> MSASFVPNGASLEDCHCNLFCLADLTGIKWKKYVWQGPTSAPILFPVTEEDPILSSFSRCLKADVLGVWRRDQRPGRRELWIFWWGEDPSFADLIHHDLSEEEDGVWENGLSYECRTLLFKAVHNLLERCLMNRNFVRIGKWFVKPYEKDEKPINKSEHLSCSFTFFLHGDSNVCTSVEINQHQPVYLLSEEHITLAQQSNSPFQVILCPFGLNGTLTGQAFKMSDSATKKLIGEWKQFYPISCCLKEMSEEKQEDMDWEDDSLAAVEVLVAGVRMIYPACFVLVPQSDIPTPSPVGSTHCSSSCLGVHQVPASTRDPAMSSVTLTPPTSPEEVQTVDPQSVQKWVKFSSVSDGFNSDSTSHHGGKIPRKLANHVVDRVWQECNMNRAQNKRKYSASSGGLCEEATAAKVASWDFVEATQRTNCSCLRHKNLKSRNAGQQGQAPSLGQQQQILPKHKTNEKQEKSEKPQKRPLTPFHHRVSVSDDVGMDADSASQRLVISAPDSQVRFSNIRTNDVAKTPQMHGTEMANSPQPPPLSPHPCDVVDEGVTKTPSTPQSQHFYQMPTPDPLVPSKPMEDRIDSLSQSFPPQYQEAVEPTVYVGTAVNLEEDEANIAWKYYKFPKKKDVEFLPPQLPSDKFKDDPVGPFGQESVTSVTELMVQCKKPLKVSDELVQQYQIKNQCLSAIASDAEQEPKIDPYAFVEGDEEFLFPDKKDRQNSEREAGKKHKVEDGTSSVTVLSHEEDAMSLFSPSIKQDAPRPTSHARPPSTSLIYDSDLAVSYTDLDNLFNSDEDELTPGSKKSANGSDDKASCKESKTGNLDPLSCISTADLHKMYPTPPSLEQHIMGFSPMNMNNKEYGSMDTTPGGTVLEGNSSSIGAQFKIEVDEGFCSPKPSEIKDFSYVYKPENCQILVGCSMFAPLKTLPSQYLPPIKLPEECIYRQSWTVGKLELLSSGPSMPFIKEGDGSNMDQEYGTAYTPQTHTSFGMPPSSAPPSNSGAGILPSPSTPRFPTPRTPRTPRTPRGAGGPASAQGSVKYENSDLYSPASTPSTCRPLNSVEPATVPSIPEAHSLYVNLILSESVMNLFKDCNFDSCCICVCNMNIKGADVGVYIPDPTQEAQYRCTCGFSAVMNRKFGNNSGLFLEDELDIIGRNTDCGKEAEKRFEALRATSAEHVNGGLKESEKLSDDLILLLQDQCTNLFSPFGAADQDPFPKSGVISNWVRVEERDCCNDCYLALEHGRQFMDNMSGGKVDEALVKSSCLHPWSKRNDVSMQCSQDILRMLLSLQPVLQDAIQKKRTVRPWGVQGPLTWQQFHKMAGRGSYGTDESPEPLPIPTFLLGYDYDYLVLSPFALPYWERLMLEPYGSQRDIAYVVLCPENEALLNGAKSFFRDLTAIYESCRLGQHRPVSRLLTDGIMRVGSTASKKLSEKLVAEWFSQAADGNNEAFSKLKLYAQVCRYDLGPYLASLPLDSSLLSQPNLVAPTSQSLITPPQMTNTGNANTPSATLASAASSTMTVTSGVAISTSVATANSTLTTASTSSSSSSNLNSGVSSNKLPSFPPFGSMNSNAAGSMSTQANTVQSGQLGGQQTSALQTAGISGESSSLPTQPHPDVSESTMDRDKVGIPTDGDSHAVTYPPAIVVYIIDPFTYENTDESTNSSSVWTLGLLRCFLEMVQTLPPHIKSTVSVQIIPCQYLLQPVKHEDREIYPQHLKSLAFSAFTQCRRPLPTSTNVKTLTGFGPGLAMETALRSPDRPECIRLYAPPFILAPVKDKQTELGETFGEAGQKYNVLFVGYCLSHDQRWILASCTDLYGELLETCIINIDVPNRARRKKSSARKFGLQKLWEWCLGLVQMSSLPWRVVIGRLGRIGHGELKDWSCLLSRRNLQSLSKRLKDMCRMCGISAADSPSILSACLVAMEPQGSFVIMPDSVSTGSVFGRSTTLNMQTSQLNTPQDTSCTHILVFPTSASVQVASATYTTENLDLAFNPNNDGADGMGIFDLLDTGDDLDPDIINILPASPTGSPVHSPGSHYPHGGDAGKGQSTDRLLSTEPHEEVPNILQQ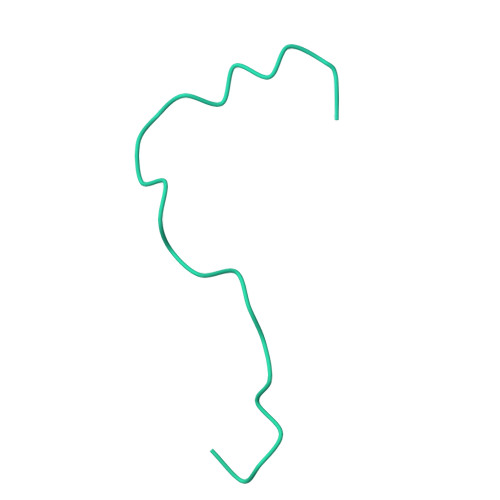PLALGYFVSTAKAGPLPDWFWSACPQAQYQCPLFLKASLHLHVPSVQSDELLHSKHSHPLDSNQTSDVLRFVLEQYNALSWLTCDPATQDRRSCLPIHFVVLNQLYNFIMNML> MFNIGA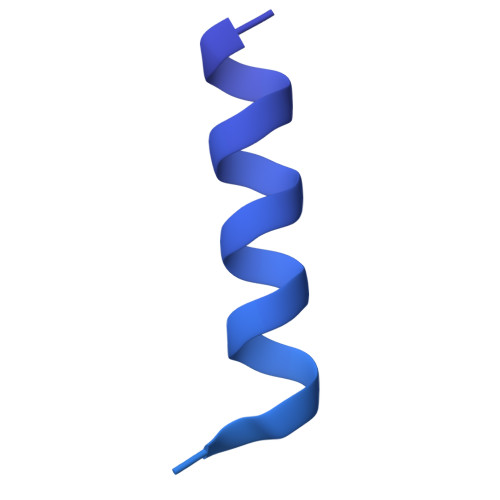GEMVFILVAALLILGPQRLPELARGIGKFLREFRRQTDEVRNVVEREFYAMDQEIGEPPTAPLRPGTRFAPQPPQAVGGPEATLPPATDGASPPADAASPQPSSPAQVLEMDAQGPREVATSDVHAGETPAQDAATAEPGAEPTAEAPPEPAASTATSPTLSPIPGTVARNAPKRSWSHPQFEK>[4x]GSMHHHHHHMNQLTILEAGLDEIICETVPGEAIQYSRYSLDRTSPLAGGCAWIEGAFVPAAAARISIFDAGFGHSDVTYTVAHVWHGNFFRLEDHVERFLAGAEKMRIPMPATKAEIMDLMRGCVSKSGLREAAVNVCVTRGYGRKPGEKTLEALESQLYVYAIPYLWVFSPIRQIEGIDAVIAQSVRRSPANVMDPWIKNYQWGDLVRATFEAQERGARTAFLLDS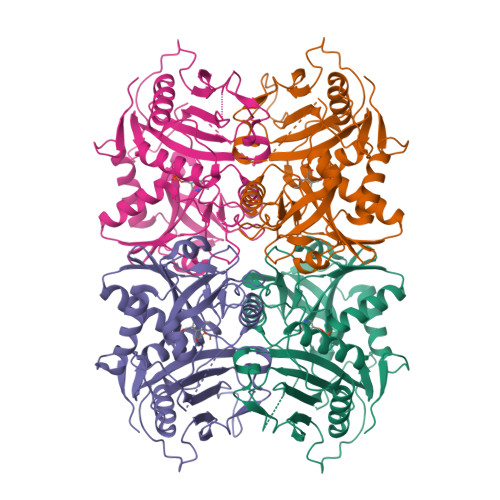DGFVTEGPGFNVLMVKDGTVFTAARNVLPGITRRTALEIARDFGLQTVIGDVTPEMLRGADEIFAATTAGGVTPVVALDGAPVGAGVPGDWTRKIRTRYWQMMDEPSDLIEPVSYI>QRMEGNGPAAVHYQPASPPRDACVYSSCYSEENVWKLCEYIKNHDQYPLEECYAVFISNERKMIPIWKQQARPGDGPVIWDYHVVLLHVSSGGQSFIYDLDTVLPFPCLFDTYVEDAIKSDDDIHPQFRRKFRVICADSYLKNFASDRSHMKDSSGNWREPPPPYPCIETGDSKMNLNDFISMDPKVGWGAVYTLSEFT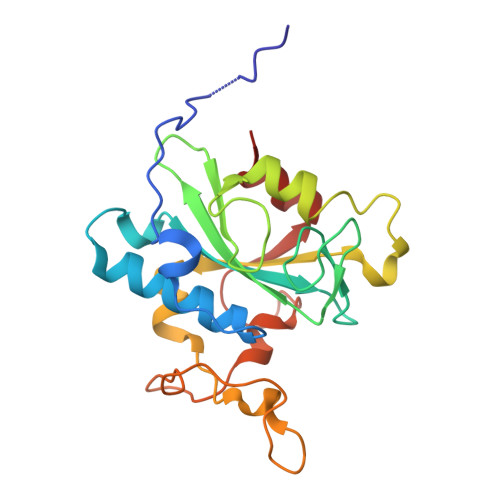HRFGS[2x]1-cyano-2-(2-methylbutan-2-yl)-3-pyridin-3-yl-guanidine | C12 H17 N5 | 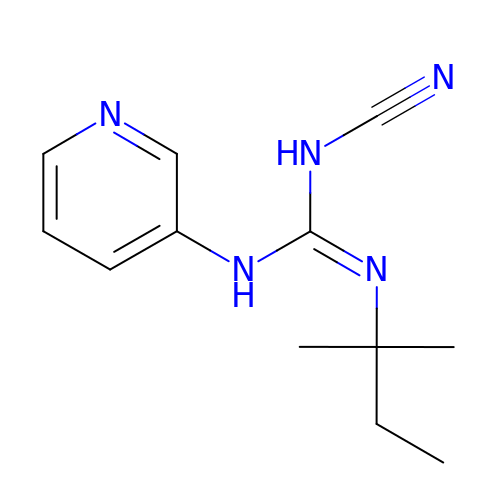HKZNADVVGXKQDL-UHFFFAOYSA-N4-({2-[(3R)-3-aminopiperidin-1-yl]-3-(but-2-yn-1-yl)-4-oxo-3,4-dihydro-5H-imidazo[2,1-b]purin-5-yl}methyl)benzonitrile 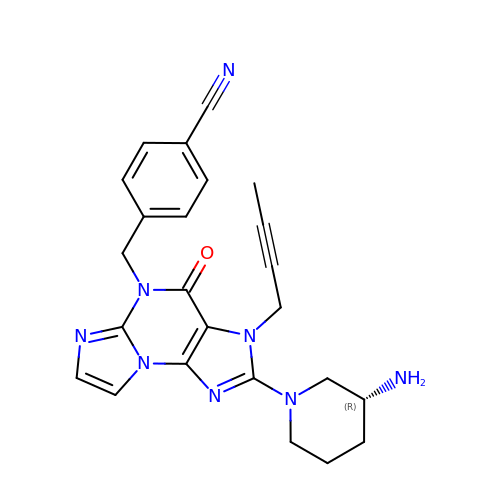| C24 H24 N8 O | KWDNXNYGKOAJBG-LJQANCHMSA-N> 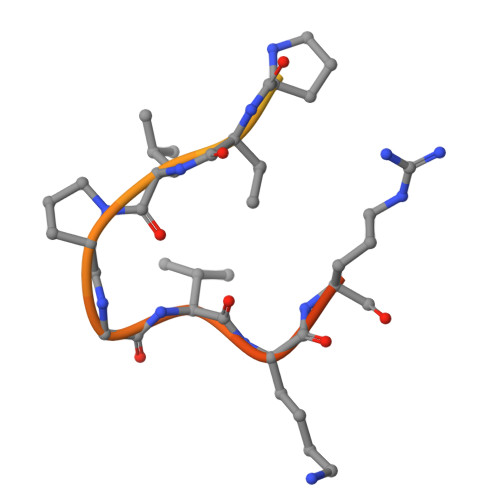RSFYTASPLLSSGSIPKSASPVLPGVKRTASVR> MAAQGFLLIATFLLVLMVLARPLGSGLARLINDIPLPGTTGVERVLFRALGVSDREMNWKQYLCAILGLNMLGLAVLFFMLLGQHYLPLNPQQLPGLSWDLALNTAVSFVTNTNWQSYSGETTLSYFSQMAGLTVQNFLSAASGIAVIFALIRAFTRQSMSTLGNAWVDLLRITLWVLVPVALLIALFFIQQGALQNFLPYQAVNTVEGAQQLLPMGPVASQEAIKMLGTNGGGFFNANSSHPFENPTALTNFVQMLAIFLIPTALCFAFGEVMGDRRQGRMLLWAMSVIFVICVGVVMWAEVQGNPHLLALGTDSSINMEGKESRFGVLVSSLFAVVTTAASCGAVIAMHDSFTALGGMVPMWLMQIGEVVFGGVGSGLYGMMLFVLLAVFIAGLMIGRTPEYLGKKIDVREMKLTALAILVTPTLVLMGAALAMMTDAGRSAMLNPGPHGFSEVLYAVSSAANNNGSAFAGLSANSPFWNCLLAFCMFVGRFGVIIPVMAIAGSLVSKKSQAASSGTLPTHGPLFVGLLIGTVLLVGALTFIPALALGPVAEYLS;> MSRKQLALFEPTLVVQALKEAVKKLNPQAQWRNPVMFIVWIGSLLTTCISIAMASGAMPGNALFSAAISGWLWITVLFANFAEALAEGRSKAQANSLKGVKKTAFARKLREPKYGAAADKVPADQLRKGDIVLVEAGDIIPCDGEVIEGGASVDESAITGESAPVIRESGGDFASVTGGTRILSDWLVIECSVNPGETFLDRMIAMVEGAQRRKTPNEIALTILLIALTIVFLLATATLWPFSAWGGNAVSVTVLVALLVCLIPTTIGGLLSAIGVAGMSRMLGANVIATSGRAVEAAGDVDVLLLNKTGTITLGNRQASEFIPAQGVD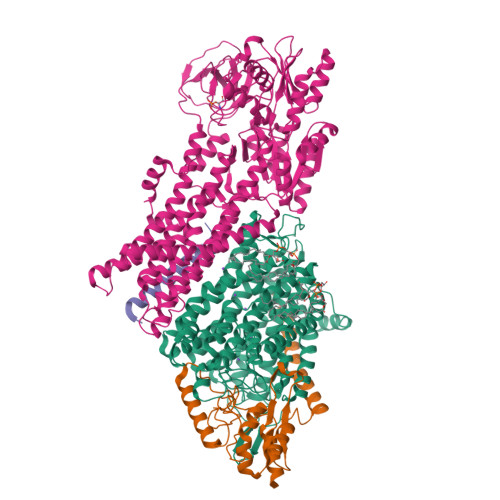EKTLADAAQLASLADETPEGRSIVILAKQRFNLRERDVQSLHATFVPFTAQSRMSGINIDNRMIRKGSVDAIRRHVEANGGHFPTDVDQKVDQVARQGATPLVVVEGSRVLGVIALKDIVKGGIKERFAQLRKMGIKTVMITGDNRLTAAAIAAEAGVDDFLAEATPEAKLALIRQYQAEGRLVAMTGDGTNDAPALAQADVAVAMNSGTQAAKEAGNMVDLDSNPTKLIEVVHIGKQMLMTRGSLTTFSIANDVAKYFAIIPAAFAATYPQLNALNIMCLHSPDSAILSAVIFNALIIVFLIPLALKGVSYKPLTASAMLRRNLWIYGLGGLLVPFIGIKVIDLLLTVCGLV;> MSGLRPALSTFIFLLLITGGVYPLLTTVLGQWWFPWQANGSLIREGDTVRGSALIGQNFTGNGYFHGRPSATAEMPYNPQASGGSNLAVSNPELDKLIAARVAALRAANPDASASVPVELVTASASGLDNNITPQAAAWQIPRVAKARNLSVEQLTQLIAKYSQQPLVKYIGQPVVNIVELNLALDKLDE;> MSAGVITGVLLVFLLLGYLVYALINAE>[4x]SATSAHSFTGRPLHIPPLPCPFPSEINEHADAVDEESHTWLAASHMLKGADTVEHFRRSKIGTLAARTNPTVPRDSLRLINDWYNWLFAFDDAFCEGELMGHRASALARALPPLLEILDG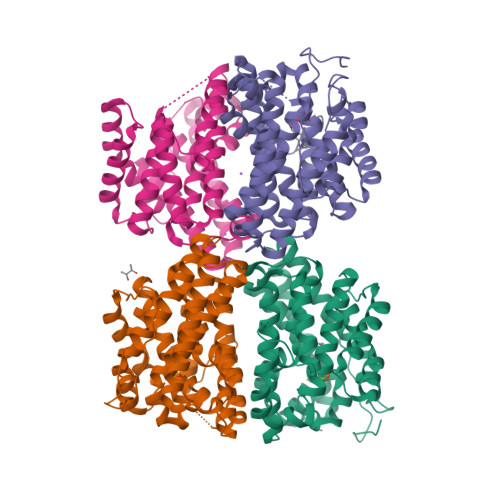RREPDGSDAFGLALKELLHRISDVASPAQVDRWRTTVKEYLFAQIWEAANREVDLIPTPDDYVLMRRITGATYTCFALIDVGGGYRLEAEEWHHPDVRTLSDLACDLIGWDNDLLSYAKERGNDKARHNLVTVLATHKSLTLQDALLEVAQMHNDAVAAFLDRRAALDRWATLPVRKYVRGLEHWVRGHIAFSLGSARYVGAWPDDTRWPRAV> MIGYLFGNRVLVD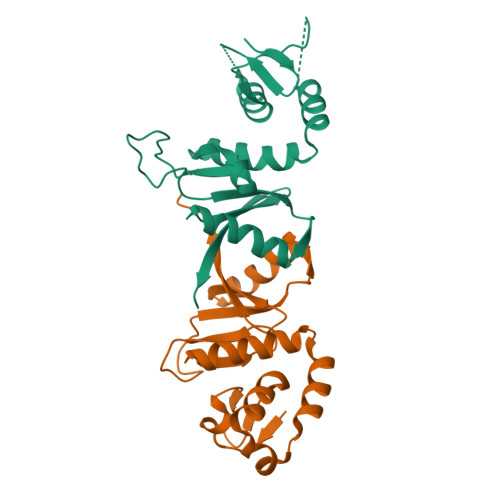DKELPLIEAYYLLDKGELEVYEDDKKLSKEEFLKKCLTYDERFLIRYKAYKELRDKGYTLGTALKFGADFRVYDIGVIPKKGKRSEREHSKWVLYPVSKDETFDFYEFASKNRVAHSTRKKMLMGIVSDKIEFIEVSWKKP;> MNLRIPWKEVYYLGYNMGNYIKISEPELLFVLRNKPQIKDRLKLDEKTIIKEGVKKYKNFWEIYYTVKDLILRGYRVRFDGFFIELYEKGIIPGTIEQDYLVYPVSGEIRMTWGELLDIYNKAIARKSKFMLAIVDSEGDVTYYEFRKLRSNK>[2x]MASQGPGEVVLLDFAAAGGELGWLTHPYGKGWDLMQNIMN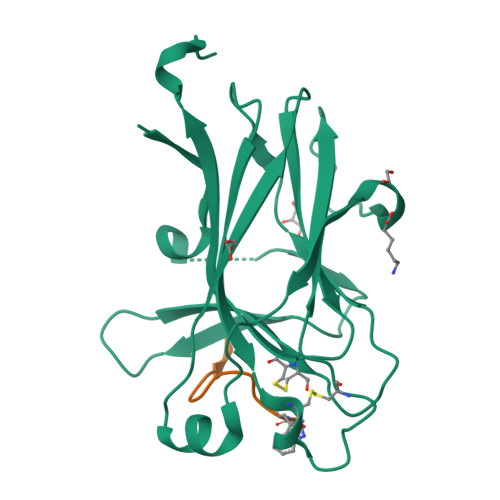DMPIYMYSVCNVMSGDQDNWLRTNWVYRGEAERIFIELKFTVRDCNSFPGGASSCKETFNLYYAESDLDYGTNFQKRLFTKIDTIAPDEITVSSDFEARHVKLNVEERSVGPLTRKGFYLAFQDIGACVALLSVRVYYKKAHHHHHH;>[2x]XWLAYPDSVPYX> SNNWDSHYGFDKAGEFHMLDHTGFAFPSEVVNGRRVLKTTDNNCWVNVTCLQLQFARFRFKSAGLQAMWESYCTGDVAMFVHWLYWLTGVDKGQPSDSENAL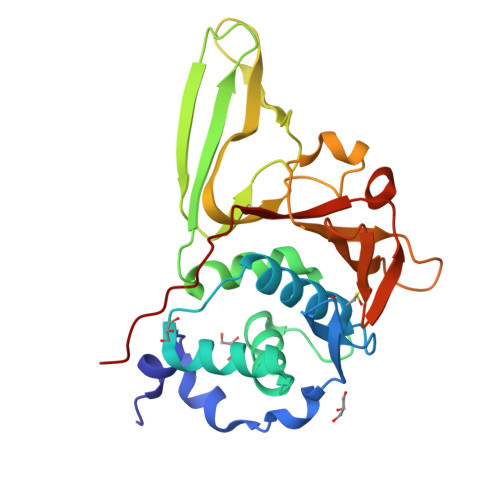NMLSKYIVPAGSVTIERVTHDGCCCSKRVVTAPVVNASVLKLGVEDGLCPHGLNYIDKVVVVKGTTIVVNVGKPVVAPSHLFLKGVSYTTFLDNGNGVAGHYTVFDHDTGMVHDGDVFVPGDLNVSPVTNVVVSEQTAVVIKDPVK1-[[4-(1,3-benzothiazol-2-yloxy)phenyl]methyl]piperidine-4-carboxylic acid | C20 H20 N2 O3 S | 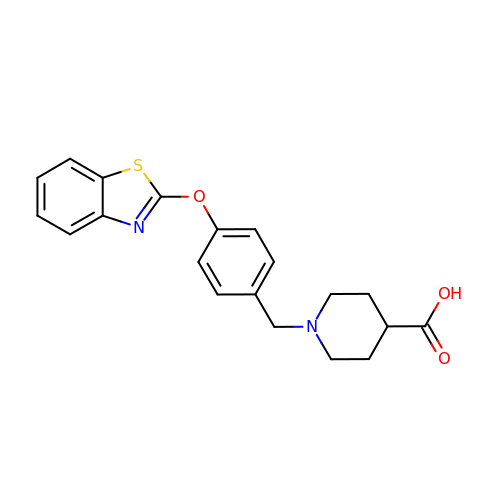BUZBVOKDNAZIIM-UHFFFAOYSA-N>MSEAAHVLITGAAGQIGYILSHWIASGELYGDRQVYLHLLDIPPAMNRLTALTMELEDCAFPHLAGFVATTDPKAAFKDIDCAFLVASMPRKPGQVRADLISSNSVIFKNTGEYLSKWAKPSVKVLVIGNPDNTNCEIAMLHAKNLKPENFSSLSMLDQNRAYYEVASKLGVDVKDVHDIIVWGNHGESMVADLTQATFTKEGKTQKVVDVLDHDYVFDTFFKKIGHRAWDILEHRGFTSAASPTKAAIQHMKAWLFGTAPGEVLSMGIPVPEGNPYGIKPGVVFSFPCNVDKEGKIHVVEGFKVNDWLREKLDFTEKDLFHEKEIALNH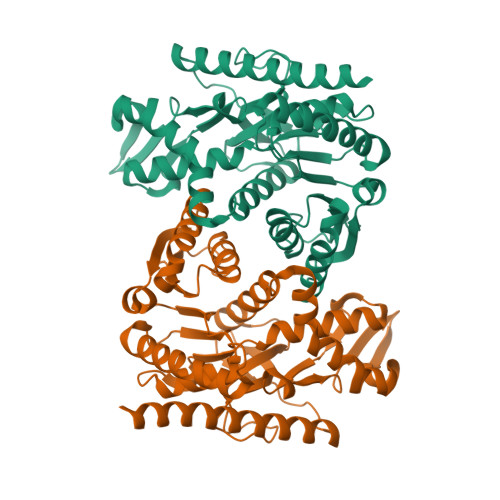LAQLEHHHHHH[2x]>RKDPIILIPSAASSILTVANIKQFLLESKYVNPRNLPSVPNGLVNIEKNFERISRPIRFIIVDNTRMFTKPEYWDRVVAIFTTGHTWQFNNYQWNSPQELFQRCKGYYFHFAGDSVPQHVQQWNVEKVELDKNKRFKDVEVVR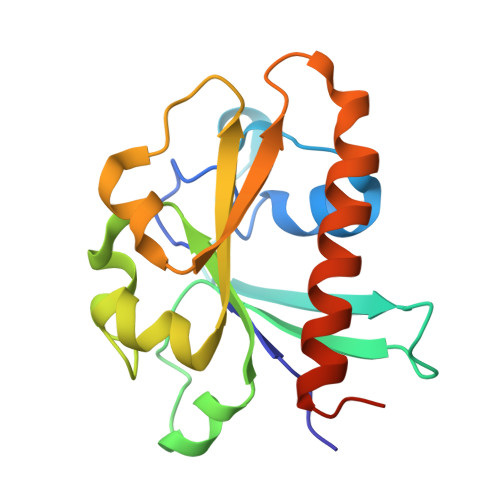YFWHSLEKELISRGYRLEHHHHHH[2x]> NGDRLYRADSRPPDEIKRSGGLMPRGHNEYFDRGTQMNINLYDHARGTQT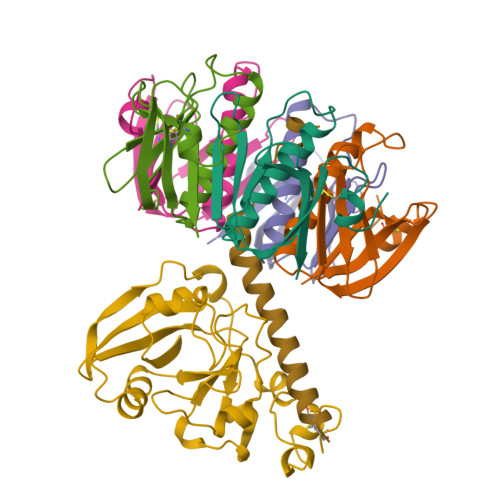GFVRYDDGYVSTSLSLRSAHLAGQSILSGYSTYYIYVIATAPNMFNKNDVLGVYSPHPYEQEVSALGGIPYSQIYGWYRVNFGVIDERLHRNREYRDRYYRNLNIAPAEDGYRLAGFPPDHQAWREEPWIHHAPQGCGNSS;> RTITGDTCNEETQNLSTIYLREYQSKVKRQIFSDYQSEVDIYNRIRDEL;>[5x]APQTITELCSEYRNTQIYTINDKILSYTESMAGKREMVIITFKSGETFQVEVPGSQHIDSQKKAIERMKDTLRITYLTETKIDKLCVWNNKTPNSIAAISMKN>[4x]SNAMIKVVFMGTPDFSVPVLRRLIED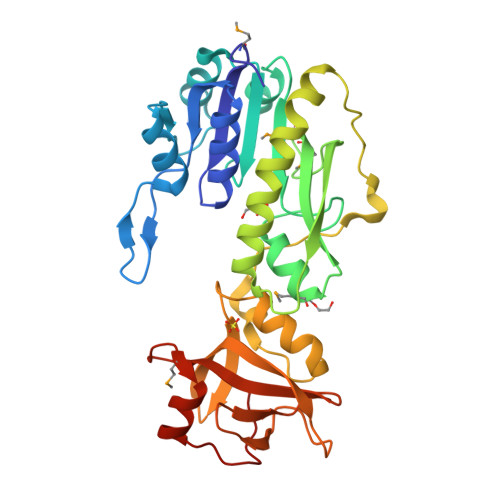GYDVIGVVTQPDRPVGRKKVLTPTPVKVEAEKHGIPVLQPLRIREKDEYEKVLALEPDLIVTAAFGQIVPNEILEAPKYGCINVHASLLPELRGGAPIHYAIMEGKEKTGITIMYMVEKLDAGDILTQVEVEIEERETTGSLFDKLSEAGAHLLSKTVPLLIQGKLEPIKQNEEEVTFAYNIKREQEKIDWTKTGEEVYNHIRGLNPWPVAYTTLAGQVVKVWWGEKVPVTKSAEAGTIVAIEEDGFVVATGNETGVKITELQPSGKKRMSCSQFLRGTKPEIGTKLGENA>GSPPWRGRREQCLLPPEDSRLWQYLLSRSMREHPALRSLRLLTLEQPQGDSMMTCEQAQLLANLARLIQAKKALDLGTFTGYSALALALALPADGRVVTCEVDAQPPELGRPLWRQAEAEHKIDLRLKPALETLDELLAAGEAGTFDVAVVDADKENCSAYYERCLQLLRPGGILAVLRVLWRGKVLQPPKG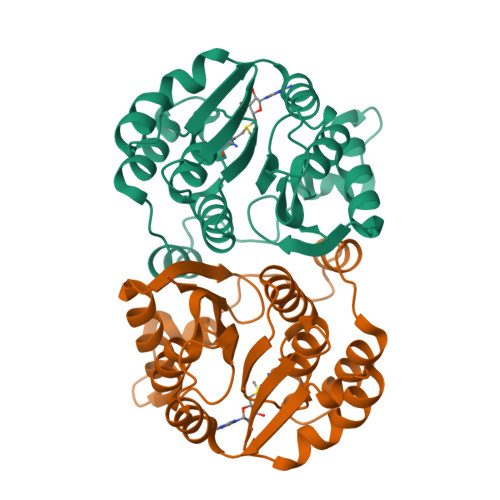DVAAECVRNLNERIRRDVRVYISLLPLGDGLTLAFKI[2x]The Aurora kinases A, B and C are serine/threonine kinases involved in the regulation of the cell division process. Aurora A is involved in the transition from the G2 to the M phase of the cell cycle by promoting centrosome maturation and mitotic spindle development. Dysfunction or overexpression of Aurora kinases has been observed in various human tumors, such as breast, lung, ovarian, prostate and colon cancer. The resulting 7-(2-anilinopyrimidin-4-yl)-1-benzazepin-2-ones were synthesized and proved to be dual inhibitors of Aurora A kinase and VEGF receptor kinases.

To confirm the binding mode of the members of the new Aurora A inhibitor class, we determined the crystal structures of the kinase in complex with the representative inhibitors 2a and 2c. The two cocrystallized inhibitors shared similar binding modes, which were in agreement with the ones suggested by the docking analyses employing the constraint between the aniline NH and Ala213 of the protein. While the anilinopyrimidine elements of the inhibitors adopted flat configurations in the ATP adenine binding pocket, the benzazepine-2-one partial structures filled the hydrophobic region. Towards the hinge area, the pyrimidine ring formed a weak hydrogen bond from C(6)H to Glu211. Another hydrogen bond was detected between the carbonyl group of Ala213 and the NH group of the aniline element. The third contact was established between the pyrimidine nitrogen atom 1 and the NH group of Ala213. In the structure with 2c, an additional interaction between the methoxy group of the ligand and Arg137 was observed. The main result drawn from the docking studies and the crystal structure analyses was the finding that the 3- and 4-positions of the aniline ring are oriented towards the entrance of the ATP binding pocket. Therefore, these positions were assumed as suitable attachment points for further substituents that would not interfere unfavorably with binding.

> GAMESKKRQWALEDFEIGRPLGKGKFGNVYLAREKQSKFILALKVLFKAQLEKAGVEHQLRREVEIQSHLRHPNILRLYGYFHDATRVYLILEYAPLGTVYRELQKLSKFDEQRTATYITELANALSYCHSKRVIHRDIKPENLLLGSAGELKIADFGWSVHAPSSRRTTLCGTLDYLPPEMIEGRMHDEKVDLWSLGVLCYEFLVGKPPFEANTYQETYKRISRVEFTFPDFVTEGARDLISRLLKHNPSQRPMLREVLEHPWITANSSKPSNCQNKESASKQS Here, we biochemically and structurally characterize a two-component defense system DUF4297–HerA, demonstrating that DUF4297–HerA confers resistance against phage infection by cooperatively cleaving dsDNA and hydrolyzing ATP. DUF4297 encodes a protein containing an N-terminal DUF4297 domain (a putative PD-(D/E)xK-family nuclease) with predicted yet-to-be biochemically characterized nuclease activity and a C-terminal domain (CTD) with unknown function. HerA, widely distributed in archaea and bacteria, encodes a DNA motor protein, which can hydrolyze ATP and translocate along DNA. The enzymatic activities and anti-phage defense function of the DUF4297–HerA system are activated through supramolecular assembly.

We incubated a 59-bp synthetic duplex DNA (dsDNA) and ATP analogs (AMPPNP or ATPγS) with purified DUF4297–HerA complex and determined three high-resolution cryo-EM structures. Particles in the sample with ATPγS generated a consensus reconstruction essentially identical to state 1. For state 1, subunit F and DNA-engaged subunit E bind the ADP molecule, whereas three other DNA-engaged subunits B–D bind the ATP molecule (AMPPNP or ATPγS in the structures). Interestingly, subunit A, which is located at the lowest position of the spiral staircase, can bind either ATP (ATPγS in the structure) or ADP molecule, suggesting that this site may be the nucleotide exchange or ATP loading position. The presence of ADP in the ATP-binding pocket can be explained by the low AMPPNP and ATPγS hydrolysis activity of the complex. Specifically, in the dataset of the sample with ATPγS and DNA, non-alignment 3D classification revealed two distinct classes with almost equal particle populations, with three densities adopting more-or-less C3 symmetry. Superimposition of these two classes showed that the linkers connecting the N-terminal DUF4297 domain and the CTD display different conformations. Further particle symmetry expansion and focused local refinement yielded two maps with an overall resolution of ~4.2 Å. The two maps align well, indicating that the DUF4297 domains in these two classes adopt a similar conformation. Two AlphaFold2-predicted DUF4297 domains fit nicely into the density, revealing dimerization of the N-terminal DUF4297 domain of the upper layer DUF4297 proteins.

>[6x]MSRNNDINAEVVSVSPNKLKISVDDLEEFKIAEEKLGVGSYLRVSDNQDVALLAIIDNFSIEVKESQKQKYMIEASPIGLVKNGKFYRGGDSLALPPKKVEPAKLDEIISIYSDSIDINDRFTFSSLSLNTKVSVPVNGNRFFNKHIAIVGSTGSGKSHTVAKILQKAVDEKQEGYKGLNNSHIIIFDIHSEYENAFPNSNVLNVDTLTLPYWLLNGDELEELFLDTEANDHNQRNVFRQAITLNKKIHFQGDPATKEIISFHSPYYFDINEVINYINNRNNERKNKDNEHIWSDEEGNFKFDNENAHRLFKENVTPDGSSAGALNGKLLNFVDRLQSKIFDKRLDFILGEGSKSVTFKETLETLISYGKDKSNITILDVSGVPFEVLSICVSLISRLIFEFGYHSKKIKRKSNENQDIPILIVYEEAHKYAPKSDLSKYRTSKEAIERIAKEGRKYGVTLLLASQRPSEISETIFSQCNTFISMRLTNPDDQNYVKRLLPDTVGDITNLLPSLKEGEALIMGDSISIPSIVKIEKCTIPPSSIDIKYLDEWRKEWVDSEFDKIIEQWSKS;>MDRSAVDTIRGYCYQVDKTIIEIFSLPQMDDSIDIECIEDVDVYNDGHLTAIQCKYYESTDYNHSVISKPIRLMLSHFKDNKEKGANYYLYGHYKSGQEKLTLPLKVDFFKSNFLTYTEKKIKHEYHIENGLTEEDLQAFLDRLVININAKSFDDQKKETIQIIKNHFQCEDYEAEHYLYSNAFRKTYDISCNKKDRRIKKSDFVESINKSKVLFNIWFYQYEGRKEYLRKLKESFIRRSVNTSPYARFFILEFQDKTDIKTVKDCIYKIQSNWSNLSKRTDRPYSPFLLFHGTSDANLYELKNQLFNEDLIFTDGYPFKGSVFTPKMLIEGFSNKEIHFQFINDIDDFNETLNSINIRKEVYQFYTENCLDIPSQLPQVNIQVKDFADIKEIV[12x]>SHMKLITAIVKPFTLDDVKTSLEDAGVLGMTVSEIQGYGRQKGHTEVYRGAEYSVDFVPKVRIEVVVDDSIVDKVVDSIVR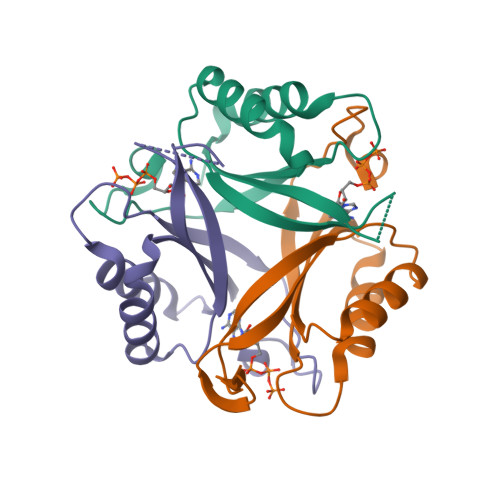AARTGKIGDGKVWVSPVDTIVRVRTGERGHDAL[3x]>[2x]SSTSLLFEQLNFLILVAAEAELPIAHSTRKLLMDNSCNNCQIYELYNENLKDVKTDKDWFMNKFGPQTVHFVISNTINFPFYKIVYFDLLIPVVSHTWVQDSVKTKRHLRTNMYSPNPFHLLRDCQVYISKSSFNKCEYILYSDLLHLLGGTLVNYISNRTTHVIVQSPQDPIIATVSKLTFGSFSSSSTNKHTEKPLREWKFVYPIWILYHFKMAKPLKGELATLCELDMQDTSEEQLFAKWEEVIGDKQTSSSQLTLHP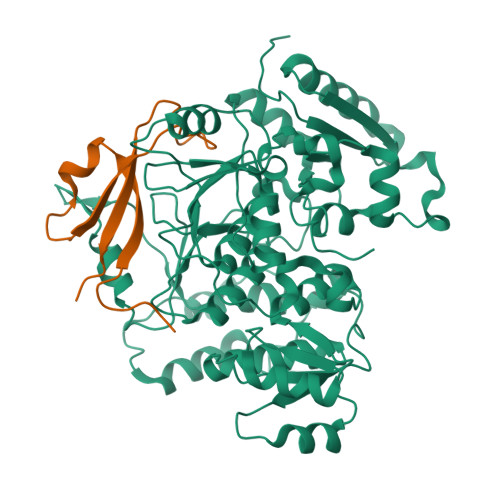NKTLFKNHHFAISPDLNFFTPLYWFLKGFIEDLDGKVTPLSFSDDLKSVYQAFPDIDCYIGHSANSPILEKTKSIKPEIHVGNVSWLFYMFALQKFTPVSQCKLIHQPFHAKLFTSKELTVAYTNYFGSQRFYIQRLVEILGGLSTPELTRKNTHLITKSTIGKKFKVAKKWSLDPQNAIIVTNHMWLEQCYMNNSKLNPKDSRFQNFKLDDNMGWNIGQIGMDHSSLPTPKNLSMVTYDTQSISEKPPPTN;>[2x]GPLGSGSSIRVKLLQESVVKLNPKLVKHNFYRVEANDSEEEETEFDDQFCIADIQLVD5-methyl-3-[4-(4-{5-[(3aS,4S,6aR)-2-oxohexahydro-1H-thieno[3,4-d]imidazol-4-yl]pentyl}-1H-1,2,3-triazol-1-yl)butyl]-1,3-benzoxazol-2(3H)-one | C24 H32 N6 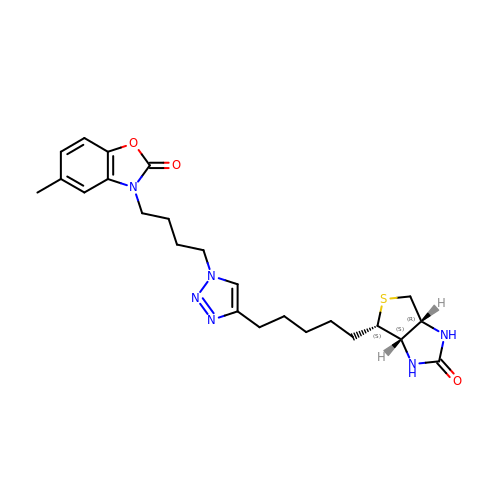O3 S | LIWDYWLHGFRYPL-NYVOZVTQSA-N> NEQLAK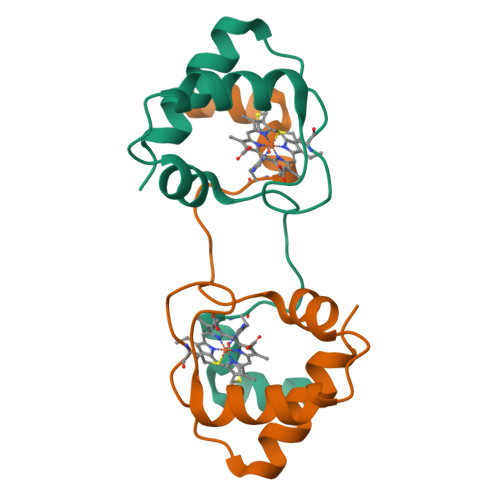QKGCMACHDLKAKKVGPAYADVAKKYAGRKDAVDYLAGKIKKGGSGVWGSVPMPPQNVTDAEAKQLAQWILSIK(3R,4R)-3-hydroxy-4-[(phosphonooxy)methyl]pyrrolidinium | C5 H13 N 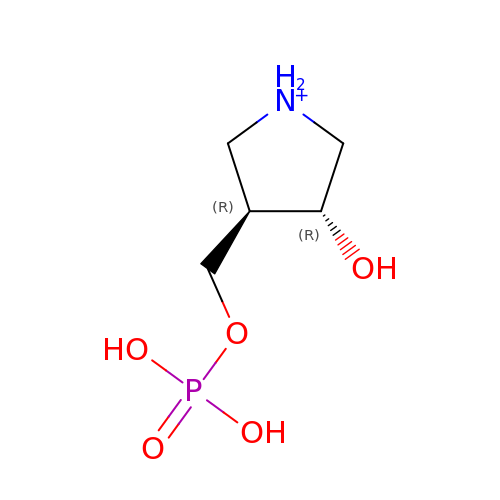O5 P | DZBMWXHITVAZTC-UHNVWZDZSA-O>GPMVEQMQQREQWCSEHLDTQKELLEEMYEEKLNILKESLTSFYQEEIQERDEKIEELEALLQEARQQSVAHQQS[2x]

The Aurora B chromosomal passenger complex (CPC) is a conserved regulator of mitosis. Aurora B localization and activation throughout mitosis and cytokinesis depend on three other proteins: INCENP, survivin, and borealin (Adams et al., 2000; 2001; Gassmann et al., 2004; Romano et al., 2003; Sampath et al., 2004; Vader et al., 2006; Wheatley et al., 2001). Together, these proteins form the tetrameric chromosomal passenger complex (CPC). MKLP2 actively promotes the movement of the CPC from chromatin to the central spindle at the onset of anaphase.

To address this question, we used a dominant-negative E413A ATPase-defective rigor mutant of MKLP2. When expressed in cells, this traps the CPC, followed using Aurora B, at an early step of the transport cycle at the boundary between chromatin and central spindle microtubules. Progressive deletion of the C terminus of MKLP2 showed that once amino acids C-terminal to position 650 are removed, Aurora B is released from this mutant MKLP2 trap. This maps the putative interaction site to a region between amino acids 650 and 750. Further fine truncation mapping defines a region close to amino acid 640–660 that is necessary to trap the CPC. Sequence alignment revealed the presence of three conserved elements within this region: an acidic patch from amino acids 636–652 that our structural analyses showed forms a paired coiled-coil elements, an invariant RRSQR sequence from amino acids 675–679, and a weakly acidic element made up of amino acids 690–705. Mutation or deletion of these three elements showed that only the first acidic patch of amino acids 636–652 was essential for interaction of the CPC with MKLP2 in anaphase. The minimal binding region of MKLP2557-668 exists in two species with molecular masses of 25.4 and 63.7 kD (yellow traces), consistent with a dimeric and a higher order oligomeric species. When mixed, CPI80 and MKLP2557-668 form a single species with a molecular mass of 100.3 kD (blue traces), consistent with two copies of CPI80 bound to a dimer of MKLP2. This proposal agrees with the dimeric structure of the core MKLP2-binding region, and dimeric structure for most known kinesin proteins.> NTVSSFQVDCFLWHVRKRFADQELGDAPFLDRLRADQASLRGRGSTLGLDIETATRAGKQIVERILEGESDEALKMPASRYLTDMTLEEMSRDWFMLMPKQK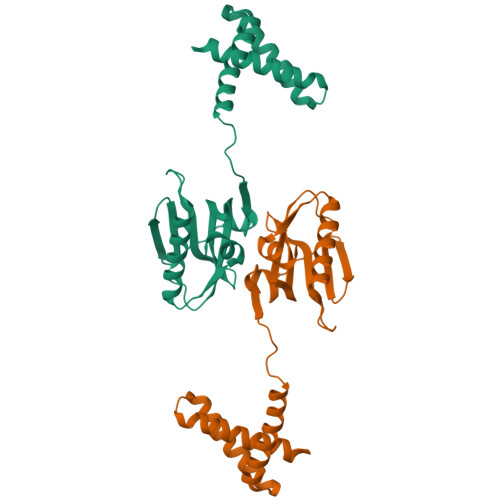VAGSLCIRMDQAIMDKNIILKANFSVIFDRLETLILLRAFTEEGAIVGEISPLPSLPGHTDEDVKNAIGVLIGGLEWNDNTVRVSETLQRFAW> GSHMPKKKIQLHAEHALYDALMILNIVKTNSPPAEEKLEDYAFNFELILEEIARLFESGDQKDEAEKAKRMKEWMKRIKTTASEDEQEEMANAIITILQSWIFS;> AVKNCSHLECFYNSRANVSCMWSHEEALNVTTCHVHAKSNLRHWNKTCELTLVRQASWACNLILGSFPESQSLTSVDLLDINVVCWEEKGWRRVKTCDFHPFDNLRLVAPHSLQVLHIDTQRCNISWKVSQ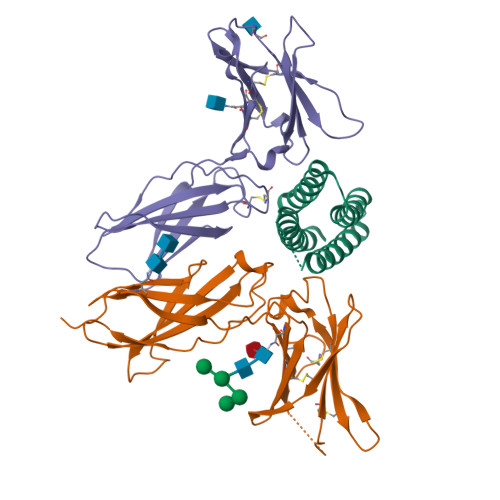VSHYIEPYLEFEARRRLLGHSWEDASVLSLKQRQQWLFLEMLIPSTSYEVQVRVKAQRNNTGTWSPWSQPLTFRTRPA;> PLPEVQCFVFNIEYMNCTWNSSSEPQATNLTLHYRYKVSDNNTFQECSHYLFSKEITSGCQIQKEDIQLYQTFVVQLQDPQKPQRRAVQKLNLQNLVIPRAPENLTLSNLSESQLELRWKSRHIKERCLQYLVQYRSNRDRSWTELIVNHEPRFSLPSVDELKRYTFRVRSRYNPICGSSQQWSKWSQPVHWGSHTVEE To further understand the structure and properties of the D:U base pair and the D:C mismatch, we designed and synthesized self-complementary RNA sequences that form duplexes with two separated or adjacent D:U or D:C pairs. All four oligonucleotides crystallized within 2–3 days at 20 °C under their optimal crystallization conditions, and we solved their structures by X-ray diffraction at a resolution higher than 1.65 Å. We found that all four structures adopt the same space group (R32). Each unit cell contains only a single RNA strand so that each duplex features two identical D-containing base pairs.

Similarly, the sequence UD-2, 5′-AGA GAA GDU CUU CUC U-3′, can form two adjacent D:U pairs with the underlined nucleobases, while the sequence CD-2, 5′-AGA GAA GDC CUU CUC U-3′, can form two adjacent D:C pairs. Examination of the crystal structures of the CD-1 and CD-2 duplexes shows that the D:C mismatches all adopt the classical wobble base pair geometry that is isomorphic with a G:U wobble pair. The N6–N3 and N1–O2 distances are similar for CD-1 and CD-2 duplexes: 2.9 Å vs 2.8 and 2.8 Å vs 2.7 Å. Based on the observed interatomic distances, the D:C pairs in the CD-1 and CD-2 duplexes appear to have two hydrogen bonds: N6–N3 and N1–O2. However, an N1–O2 hydrogen bond requires N1-protonation of D in D:C pairs. Solution-phase NMR studies revealed that the 2-aminopurine (2AP)-cytosine (C) pair exists predominantly as a protonated pair as opposed to an imino tautomer at physiological pH. Since D has an additional electron-donating amino group, N1 in D has a higher pKa value and is more likely to be protonated than N1 in 2AP. Therefore, D in the D:C pairs likely exists as a protonated D in the canonical amino tautomeric form. Crystallographic studies reveal that the protonated amino form of D can form a base pair with C that is isostructural to a G:U wobble pair, which may account for the increased rate of D:C mismatches in the defined construct. Therefore, D:C mismatches have a strong stalling effect on downstream primer extension.

> AGAGAAGGCCUUCUCU> MSVPKKRNHGKLPPSTKDVDDPSLKYTKAAPKCEQVAEHWLLQPLPEPESRYSFWVTIVTLLAFAARFYKIWYPKEVVFDEVHFGKFASYYLERSYFFDVHPPFAKMMIAFIGWLCGYDGSFKFDEIGYSYETHPAPYIAYRSFNAILGTLTVPIMFNTLKELNFRAITCAFASLLVAIDTAHVTETRLILLDAILIISIAATMYCYVRFYKCQLRQPFTWSWYIWLHATGLSLSFVISTKYVGVMTYSAIGFAAVVNLWQLLDIKAGLSLRQFMRHFSKRLNGLVLIPFVIYLFWFWVHFTVLNTSGPGDAFMSAEFQETLKDSPLSVDSKTVNYFDIITIKHQDTDAFLHSHLARYPQRYEDGRISSAGQQVTGYTHPDFNNQW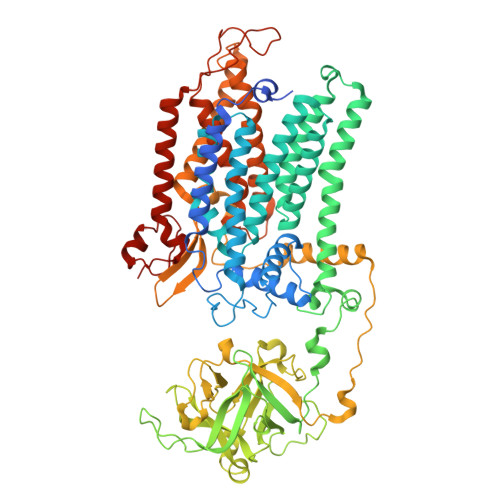EVLPPHGSDVGKGQAVLLNQHIRLRHVATDTYLLAHDVASPFYPTNEEITTVTLEEGDGELYPETLFAFQPLKKSDEGHVLKSKTVSFRLFHVDTSVALWTHNDELLPDWGFQQQEINGNKKVIDPSNNWVVDEIVNLDEVRKVYIPKVVKPLPFLKKWIETQKSMFEHNNKLSSEHPFASEPYSWPGSLSGVSFWTNGDEKKQIYFIGNIIGWWFQVISLAVFVGIIVADLITRHRGYYALNKMTREKLYGPLMFFFVSWCCHYFPFFLMARQKFLHHYLPAHLIACLFSGALWEVIFSDCKSLDLEKDEDISGASYERNPKVYVKPYTVFLVCVSCAVAWFFVYFSPLVYGDVSLSPSEVVSREWFDIELNFSK> MQSLEKQSSKGQWLTTWATAPQLVEPKNLPPEPGLSGNTLRQIVRVSVGGKKLRLRFSNKYSMDSLAVKAVSIAVPSDSSNVDAATIRSLTFEKKNNFKIAPGSDIYSDEVNFNLKPNSLLAITVSYAKVTQSVTGHPASRTTSFIVKGEQTNAEVFKNPVKTDHWYSLFNIDVKTSEPSYAVAIMGNSITDGRGSGTNRQNRWPDIFSQRLLANPSTRNISVLNLGIGGNCVVRGGLGPTALDRFDYNILNQQGVKWLIILEGVNDLGGTRDPDDASKRTEELIAAYQVMIDKAHANGIKVYGATILPFGKSFYEKPFRIEEWKKVNDWIRNSGKFDAVIDFAKHMQSENPEVILNDMHDHDFLHPNEAGYRRMGEFVDLNLFKNE

Acetyl xylan esterases (AcXE) that target mono- or doubly acetylated Xylp are well characterized; however, the previously studied AcXE from Flavobacterium johnsoniae (FjoAcXE) was the first to remove the acetyl group from 2-O-MeGlcpA-3-O-acetyl-substituted Xylp units, yet structural characteristics of these enzymes remain unspecified. All homologs were confirmed to release acetate from 2-O-MeGlcpA-3-O-acetyl-substituted xylan, and the crystal structures point to key structural elements that might serve as defining features of this unclassified carbohydrate esterase family. Enzymes comprised two domains: N-terminal CBM domain and a C-terminal SGNH domain. In FjoAcXE and all studied homologs, the sequence motif around the catalytic serine is Gly-Asn-Ser-Ile (GNSI), which differs from other SGNH hydrolases.

The crystal structure of CspAcXE was solved in the native state (1.30 Å). The sequence identity between the CspAcXE and PbeAcXE is 52.4%. Both comprise an N-terminal CBM-like domain consisting of three antiparallel β-sheets, and a C-terminal SGNH domain where the central β-sheet comprises five parallel β-strands flanked on both sides with α-helices. In both cases, the CBM-like and catalytic SGNH domains are tightly packed and connected through a loop of six to seven amino acids. The residues forming the CBM-like domains in PbeAcXE and CspAcXE are 1–175 and 1–176, respectively, whereas residues forming the SGNH domain in PbeAcXE and CspAcXE are 180–385 and 181–386, respectively. The first seven N-terminal residues of PbeAcXE and the first 10 residues of CspAcXE did not have electron density and so were not included in the final structures. Moreover, residues 350 to 365 in CspAcXE, which form a loop next to the active site, had unclear or missing electron density and so were omitted from the solved structure; this could be the result of the absence of ligand to stabilize its conformation, or due to the absence of many crystal packing contacts in this region of the protein. The Ser-Asp-His catalytic triad is formed by Ser188, Asp363, and His366 in PbeAcXE, and Ser189, Asp363, and His366 in CspAcXE. In CspAcXE, these residues are Ser189, Gly229 and Asn266. Therefore, like the GDSL-hydrolases, the GNSI-AcXEs do not have the nucleophilic elbow; this is corroborated by the crystal structures of PbeAcXE and CspAcXE, which show that the Asn in this motif (Asn187 and Asn188) are buried into the interior of the enzymes.> ETGDVKPDLQTKQDKVLAHFIGNSTDYFKILDHNDEFVLVGAKDVIYNVSLNGLKEIARLEWHSTDADRELCALKGKHEWDC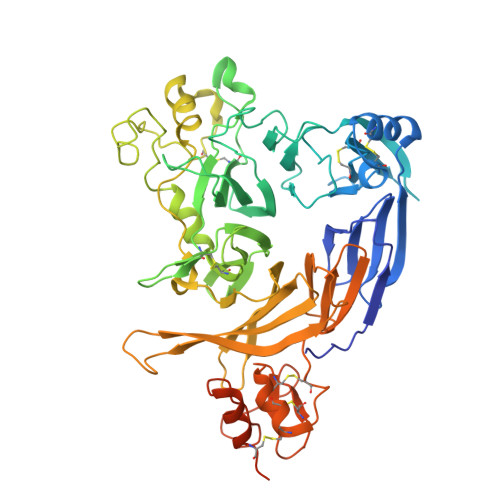HNYLRVYALRPNGEVLLCGTNSYKPRCRHYTPVEVSSEEAGSAGHAHAMRYEVSRDVEAQGLCPYSPAHNSTYAFADGHLYSATVADFSGGDPLIYRENLRTEQYDLKQLNQPDFVGAIERNGYVLFFFRELSMEVMNFGKAVYSRVARVCKNDRGGPYSHGKSWTSFLKARLNCSVPGEFPFYFDEIQAISPIVESGSKSLIYAVFTTSVNAIPGSAVCAFNVDDILAAFDGEFKSQKDSQSHWLPVEREQVPKPRPGQCVEDSRTLTSIAVNFIKNHPLMEEAVPAVHGRPLLTKVNLHHRLTAIAVHPQVKSLSGAYYDVIYSGTDDGKVTKFINILSTHPNSTVDRLKTVVISEMQVLPLGTPIRELVISTSKNSLVVVSDGSLVSVPLHHCSHIVDCLGCLSLQDPICAWDLQTHECKNLATSQHKFGTKTYLQSLNSTKKAAALLCPHIPRDAPGAETVSFVTMAPPPTEEQKLLYSNVGSGTKHHHHHH> GAMEQWCSERLDNQKELMEELYEEKLKILKESLTTFYQEQIQERDEKIEELETLLQ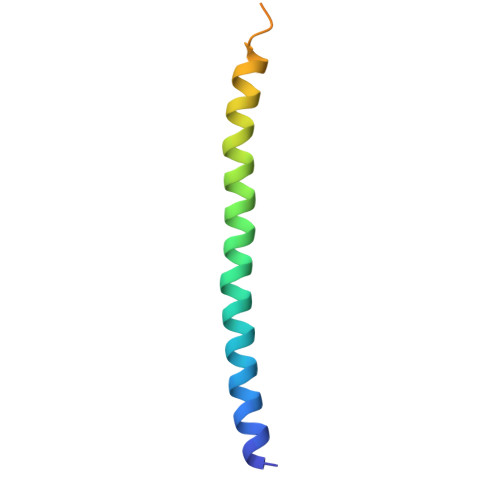EAKQQPAAQQ(2S)-1-{[(2R)-1-{[(2S,3S)-1-cyclohexyl-3-hydroxy-4-(2-oxopyridin-1(2H)-yl)butan-2-yl]amino}-3-(methylsulfanyl)-1-oxopropan-2-yl]amino}-1-oxo-3-phenylpropan-2-yl 4-aminopiperidine-1-carboxylate | C34 H49 N5 O6 S | 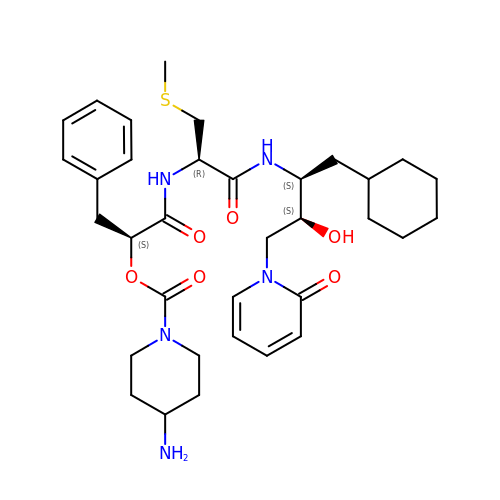HYLLVLPQGWZUHR-KRCBVYEFSA-N> MIGVNRMTEASTYIGTVQDVNGANIRVVLDINTISSLKFVDGQGYRIGQIGSFVRIPIGYINLFGIVSQVGAGAVPDKLLEVEPYGHRWISVQLVGEEGIKKEFERGVSQYPTIGDKVHIVTEPDLKKIYGTQNKKYISLGNIASVDSIPALVNIDTLVTRHSAVLGSTGSGKSTTVTSILQRISDMSQFPSARIIVFDIHGEYAAAFKGKAKVYKVTPSNNELKLSIPYWALTCDEFLSVAFGGLEGSGRNALIDKIYELKLQTLKRQEYEGINEDSLTVDTPIPFSIHKLWFDLYRAEISTHYVQGSHSEENEALLLGEDGNPVQKGD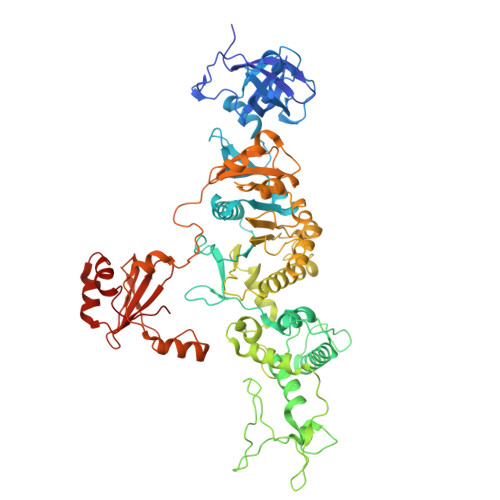SLKVVPPIYMPHTQAQGATKIYLSNRGKNIRKPLEGLASLLKDPRYEFLFNADDWSVNLDGKTNKDLDALLETWVGSEESISIFDLSGMPSSILDTLIGILIRILYDSLFWSRNQPEGGRERPLLVVLEEAHTYLGKDSRGIAIDGVRKIVKEGRKYGIGMMLVSQRPSEIDSTILSQCGTLFALRMNNSSDRNHVLGAVSDSFEGLMGMLPTLRTGEAIIIGESVRLPMRTIISPPPFGRRPDSLDPDVTAKWSNNRVQGDYKEVLTLWRQKKVRSQRIVENIKRLPVVNEGEMTDMVREMVTSSNILSIGYEADSMTLEIEFNHGLVYQYYDVPETLHTELLAAESHGKFFNSQIKNNYRFSRI>MHHHHHHENLYFQGAASMNKKTKLIHGGHTTDDYTGAVTTPIYQTSTYLQDDIGDLRQGYEYSRTANPTRSSVESVIAALENGKHGFAFSSGVAAISAVVMLLDKGDHIILNSDVYGGTYRALTKVFTRFGIEVDFVDTTHTDSIVQAIRPTTKMLFIETPSNPLLRVTDIKKSAEIAKEHGLISVVDNTFMTPYYQNPLDLGIDIVLHSATKYLGGHSDVVAGLVATSDDKLAERLAFISNSTGGILGPQDSYLLVRGIKTLGLRMEQINRSVIEIIKMLQAH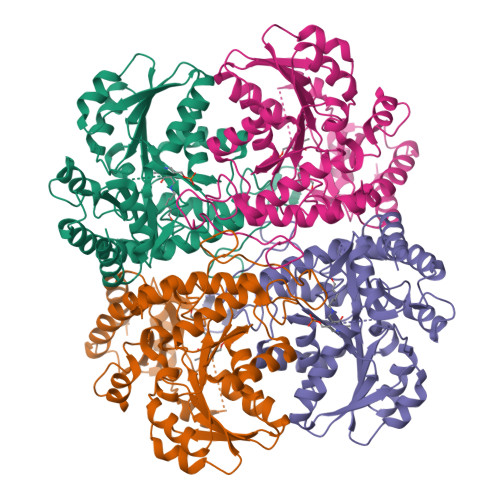PAVQQVFHPSIESHLNHDVHMAQADGHTGVIAFEVKNTESAKQLIKATSYYTLAESLGAVESLISVPALMTHASIPADIRAKEGITDGLVRISVGIEDTEDLVDDLKQALDTL[2x]>MYLSKVIIARAWSRDLYQLHQGLWHLFPNRPDAARDFLFHVEKRNTPEGCHVLLQSAQMPVSTAVATVIKTKQVEFQLQVGVPLYFRLRANPIKTILDNQKRLDSKGNIKRCRVPLIKEAEQIAWLQRKLGNAARVEDVHPISERPQYFSGDGKSGKIQTVCFEGVLTINDAPALIDLVQQGIGPAKSMGCGLLSLAPL[2x];>MSNFINIHVLISHSPSCLNRDDMNMQKDAIFGGKRRVRISSQSLKRAMRKSGYYAQNIGESSLRTIHLAQLRDVLRQKLGERFDQKIIDKTLALLSGKSVDEAEKISADAVTPWVVGEIAWFCEQVAKAEADNLDDKKLLKVLKEDIAAIRVNLQQGVDIALSGRMATSGMMTELGKVDGAMSIAHAITTHQVDSDIDWFTAVDDLQEQGSAHLGTQEFSSGVFYRYANINLAQLQENLGGASREQALEIATHVVHMLATEVPGAKQRTYAAFNPADMVMVNFSDMPLSMANAFEKAVKAKDGFLQPSIQAFNQYWDRVANGYGLNGAAAQFSLSDVDPITAQVKQMPTLEQLKSWVRNNGEA[12x];>MRSYLILRLAGPMQAWGQPTFEGTRPTGRFPTRSGLLGLLGACLGIQRDDTSSLQALSESVQFAVRCDELILDDRRVSVTGLRDYHTVLGAREDYRGLKSHETIQTWREYLCDASFTVALWLTPHATMVISELEKAVLKPRYTPYLGRRSCPLTHPLFLGTCQASDPQKALLNYEPVGGDIYSEESVTGHHLKFTARDEPMITLPRQFASREWYVIKGGMDVSQ[2x];>[2x]MNLLIDNWIPVRPRNGGKVQIINLQSLYCSRDQWRLSLPRDDMELAALALLVCIGQIIAPAKDDVEFRHRIMNPLTEDEFQQLIAPWIDMFYLNHAEHPFMQTKGVKANDVTPMEKLLAGVSGATNCAFVNQPGQGEALCGGCTAIALFNQANQAPGFGGGFKSGLRGGTPVTTFVRGIDLRSTVLLNVLTLPRLQKQFPNESHTENQPTWIKPIKSNESIPASSIGFVRGLFWQPAHIEL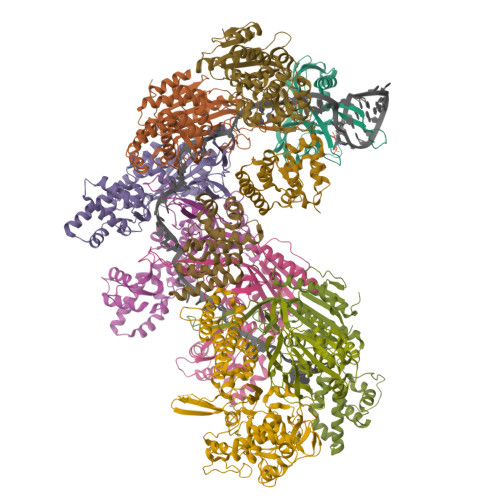CDPIGIGKCSCCGQESNLRYTGFLKEKFTFTVNGLWPHPHSPCLVTVKKGEVEEKFLAFTTSAPSWTQISRVVVDKIIQNENGNRVAAVVNQFRNIAPQSPLELIMGGYRNNQASILERRHDVLMFNQGWQQYGNVINEIVTVGLGYKTALRKALYTFAEGFKNKDFKGAGVSVHETAERHFYRQSELLIPDVLANVNFSQADEVIADLRDKLHQLCEMLFNQSVAPYAHHPKLISTLALARATLYKHLRELKPQGGPSNG;>[4x]GPGYQMADEIDAMALYRAWQQLDNGSCAQIRRVSEPDELRDIPAFYRLVQPFGWENPRHQQALLRMVFCLSAGKNVIRHQDKKSEQTTGISLGRALANSGRINERRIFQLIRADRTADMVQLRRLLTHAEPVLDWPLMARMLTWWGKRERQQLLEDFVLTTNKNA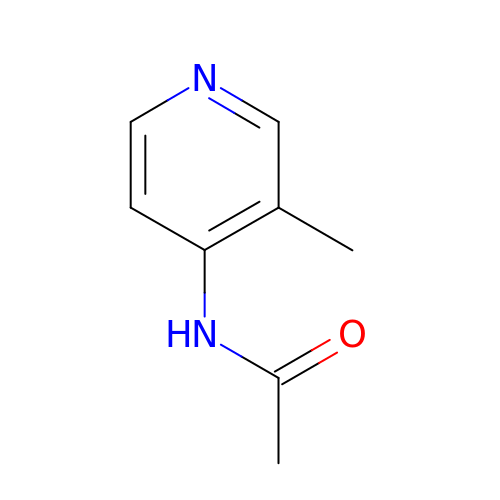N-(3-methylpyridin-4-yl)acetamide | C8 H10 N2 O | DHUDCBCQKIWLSB-UHFFFAOYSA-N> GSTGSSNRYQSYLEGVKYNVDSAIQTITKIYNTYTLFSTKLTQMYSTRLDNFAKAKAKEEAAKFTKEDLEKNFKTLLNYIQVS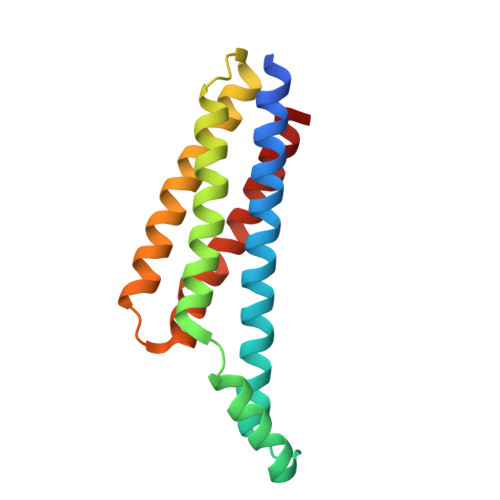VKTAANFVYINDTHAKRKLENIEAEIKTLIAKIKEQSNLYEAYKAIVTSILLMRDSLKEVQGIID(1r,1'S,3'S,5'S,7'S)-spiro[cyclohexane-1,2'-tricyclo[3.3.1.1~3,7~]decan]-4-amine 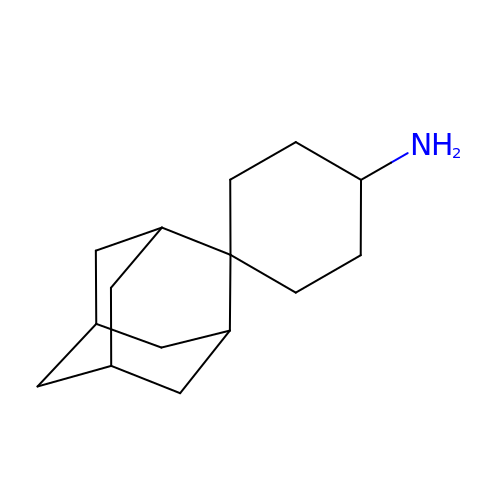| C15 H25 N | VNTMIVFMVGTSHV-RLUXGHLOSA-N> AAPAVLGEVDTSLVLSSMEEAKQLVDKAYKERRESIKQRLRSGSASPMELLSYFKQPVAATRTAVRAADYLHVALDLLERKLRSLWRRPFNVTDVLTPAQLNVLSKSSGCAYQDVGVTCPEQDKYRTITGMCNNRRSPTLGASNRAFVRWLPAEYEDGFSLPYGWTPGVKRNGFPVALARAVSNEIVRFPTDQLTPDQERSLMFMQWGQLLDHDLDFTPEPAARASFVTGVNCETSCVQQPPCFPLKIPPNDPRIKNQADCIPFFRSCPACPGSNITIRNQINALTSFVDASMVYGSEEPLARNLRNMSNQLGLLAVNQRFQDNGRALLPFDNLHDDPCLLTNRSARIPCFLAGDTRSSEMPELTSMHTLLLREHNRLATELKSLNPRWDGERLYQEARKIVGAMVQIITYRDYLPLVLGPTAMRKYLPTYRSYNDSVDPRIANVFTNAFRYGHTLIQPFMFRLDNRYQPMEPNPRVPLSRVFFASWRVVLEGGIDPILRGLMATPAKLNRQNQIAVDEIRERLFEQVMRIGLDLPALNMQRSRDHGLPGYNAWRRFCGLPQPETVGQLGTVLRNLKLARKLMEQYGTPNNIDIWMGGVSEPLKRKGRVGPLLACIIGTQFRKLRDGDRFWWENEGVFSMQQRQALAQISLPRIICDNTGITTVSKNNIFMSNSYPRDFVNCSTLPALNLASWREAS

Neutrophils figure prominently in human host defense against infection, and optimal antimicrobial action in neutrophils relies on the action of hypochlorous acid (HOCl), the product of the myeloperoxidase (MPO)4-H2O2-chloride system. In MPO, the prosthetic group is covalently linked to the protein via autocatalytic formation of two ester bonds with highly conserved aspartate and glutamate residues and a sulfonium ion linkage between the 2-vinyl group and a conserved methionine. Among members of the peroxidase-cyclooxygenase superfamily, mature MPO alone is a functional dimer, composed of two identical glycosylated protomers that contain covalently bound heme, an N-terminal 14.5-kDa light polypeptide (L-chain), and a 59-kDa heavy polypeptide (H-chain), with the two H-chains linked covalently by a single Cys-319–Cys-319 bridge. ProMPO contains a 116-amino acid N-terminal pro-region that is required for its stability, as its deletion results in retention of proMPO in the ER and failure to undergo proteolytic processing to generate mature MPO, but its precise function and fate during MPO biosynthesis are unknown.

We present the high-resolution crystal structure of proMPO recombinantly produced by CHO cells and demonstrate how the flexible propeptide blocks dimerization by the formation of a disulfide bridge between Cys-158 from the propeptide and Cys-319. Monoclinic proMPO crystals (space group C2) were grown with one proMPO molecule per asymmetric unit. Because an SDS-PAGE of the crystals demonstrated the presence of the full-length protein, this clearly suggests that the propeptide exhibits a high flexibility compared with the core of the protein (Thr-166–Ala-744). The segment of the propeptide visible in the electron density of proMPO is anchored to the core protein via a cystine bridge (Cys-158–Cys-319) together with polar and hydrophobic interactions, resulting in a buried surface area of 399 Å2. The same disulfide bridges are found in mature MPO, with Cys-167–Cys-180 located in the L-chain and the remaining disulfide bridges belong to the H-chain of leukocyte MPO. However, most interestingly, Cys-319 of proMPO, which is known to form an interchain disulfide bridge between the H-chains of the symmetry-related halves (74 kDa) in dimeric MPO (compare with Fig. 1A), formed a disulfide bridge with Cys-158 of the propeptide. The crystal structure of proMPO shows that the stretch 273ASFVTG278 was part of a surface-exposed α-helix loop segment with all six amino acids surface exposed (accessible surface areas follow the hierarchy Phe-275 > Gly-278 > Val-276 > Ala-273 > Ser-274 > Thr-277). The structure of proMPO that we reported here fully supports these findings, because it demonstrates that its core structure, including the substrate access channel and heme cavity architecture, was almost identical to that of the protomer of mature MPO.>RICFNHQS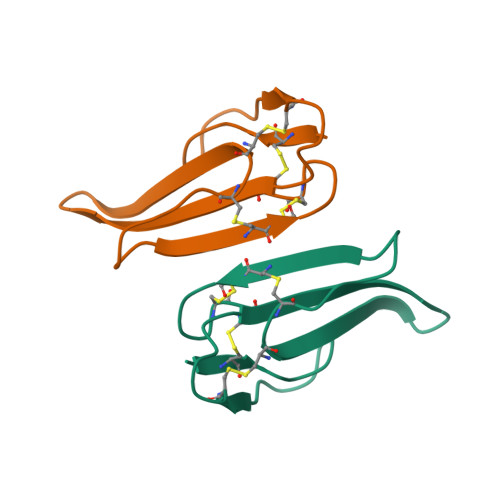SQPQTTKTCSPGESSCYHKQWSDFRGTIIERGCGCPTVKPGINLSCCESEVCNN[2x]> MFKILDWYIGRTIVATTALVLVTFVGLSGIIKYVEQLRKVGEGSYDLLQALLFVVLSIPRDVEMFFPMAALLGALIGLGALASSSELVVMQAAGFSKLDIGLSVLKTAIPLMIIVTLLGEWGA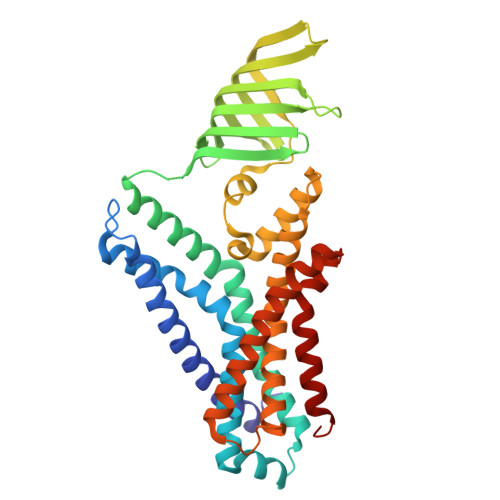PQAQKMARDMRAFATSGGAIMSVRTGVWARDANDFIFIAKVENEHLYGLNLWRFDENKKLSTVIFSEQVDYVANNEWLMKDAVLTRLVNDIEISKESLPEYRWRTSLAPDKLAVVTVKPEELSLTGLSDYVHYLKASEQDSSRYELALWRKVTQPISIAVMMLMALSFIFGPLRSVTMGARILSGVIAGFSFYISSEFFGPLSLVYGLPPLFGALAPSLVFLAIALGLLGRKL>MGKSLSHLPLHSSKEDAYDGVTSENMRNGLVNSEVHNEDGRNGDVSQFPYVEFTGRDSVTCPTCQGTGRIPRGQENQLVALIPYSDQRLRPRRTKLYVMASVFVCLLLSGLAVFFLFPRSIDVKYIGVKSAYVSYDVQKRTIYLNITNTLNITNNNYYSVEVENITAQVQFSKTVIGKARLNNISIIGPLDMKQIDYTVPTVIAEEMSYMYDFCTLISIKVHNIVLMMQVTVTTTYFGHSEQISQERYQYVDCGRNTTYQLGQSEYLNVLQPQQ[4x]

pmcAmyotrophic lateral sclerosis/parkinsonism-dementia complex (ALS/PDC or lytico-bodig) is a fatal disease found in the Chamorro population of Guam (1–4), some families on the Kii peninsula of Japan, and the Auyu and Jakai people of New Guinea. Abundant filamentous amyloid inclusions that are made of all six brain tau isoforms are characteristic of ALS/PDC. We now show that tau filaments from Guam and Kii ALS/PDC adopt the CTE fold in brain and spinal cord. The greater heterogeneity of amyloid filaments, when compared to CTE and SSPE, probably reflects the fact that ALS/PDC is a multiple proteinopathy based on neuropathology, as suggested for cases from the Kii peninsula.

In addition to tau filaments, we also observed singlets and doublets of transmembrane protein 106B (TMEM106B) filaments (fold I) in the frontal cortex from cases 1 and 2, and TMEM106B singlets (fold I) in the spinal cord from case 2. Senile plaques have been described in around 60% of cases of Guam ALS/PDC and assembly of Aβ is believed to be part of the disease process. Alternatively, these changes may be age-related. This was probably also the reason for the presence of TMEM106B filaments in two cases from Guam and one case from the Kii peninsula.(1S,4R)-2-azabicyclo[2.2.1]hept-5-en-3-one | C6 H7 N O | 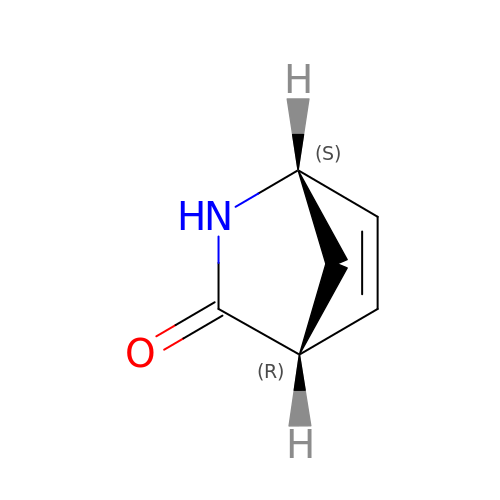DDUFYKNOXPZZIW-CRCLSJGQSA-N>[4x]MVIATDDLETTCPNCNGSG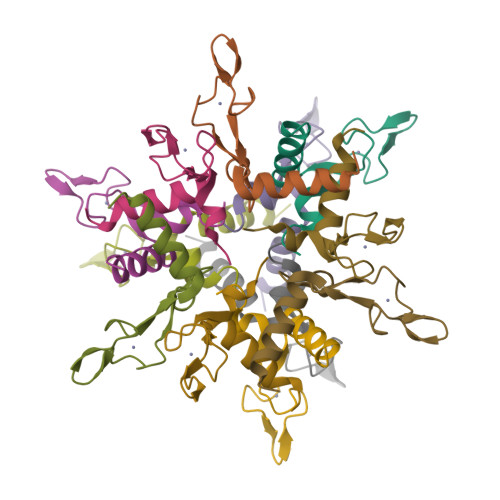REEPEPCPKCLGKGVILTAQGSTLLHFIKKHIHE>MALRVAAFDLDGVLALPSIAGAFRRSEEALALPRDFLLGAYQTEFPEGPTEQLMKGKITFSQWVPLMDESYRKSSKACGANLPENFSISQIFSQAMAARSINRPMLQAAIALKKKGFTTCIVTNNWLDDGDKRDSLAQMMCELSQHFDFLIESCQVGMIKPEPQIYNFLLDTLKAKPNEVVFLDDFGSNLKPARDMGMVTILVHNTASALRELEKVTGTQFPEAPLPVPCNPNDVSHGYVTVKPGIRLHFVEMGSGPALCLCHGFPESWFSWRYQIPALA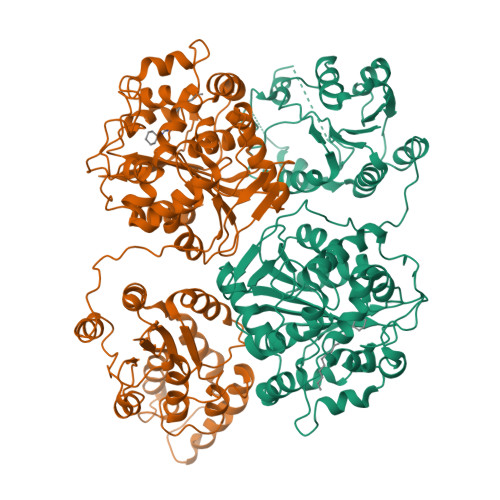QAGFRVLAIDMKGYGDSSSPPEIEEYAMELLCKEMVTFLDKLGIPQAVFIGHDWAGVMVWNMALFYPERVRAVASLNTPFMPPDPDVSPMKVIRSIPVFNYQLYFQEPGVAEAELEKNMSRTFKSFFRASDETGFIAVHKATEIGGILVNTPEDPNLSKITTEEEIEFYIQQFKKTGFRGPLNWYRNTERNWKWSCKGLGRKILVPALMVTAEKDIVLRPEMSKNMEKWIPFLKRGHIEDCGHWTQIEKPTEVNQILIKWLQTEVQNPSVTSKI[2x]> SVTSAKVAVNGVQLHYQQTGEGDHAVLLLPGMLGSGETDFGPQLKNLNKKLFTVVAWDPRGYGHSRPPDRDFPADFFERDAKDAVDLMKALKFKKVSLLGWADGGITALIAAAKYPSYIHKMVIWGANAYVTDEDSMIYEGIRDVSKWSERTRKPLEALYGYDYFARTCEKWVDGIRQFKHLPDGNICRHLLPRVQCPALIVHGEKDPLVPRFHAD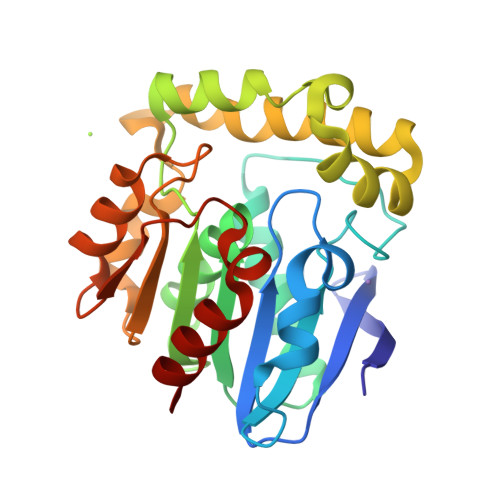FIHKHVKGSRLHLMPEGKHNLHLRFADEFNKLAEDFLQ[(2S)-3-[2-[(E)-[(2E,4E,6E,8E)-3,7-dimethyl-9-(2,6,6-trimethylcyclohexen-1-yl)nona-2,4,6,8-tetraenylidene]amino]ethoxy-oxidanyl-phosphoryl]oxy-2-[(Z)-octadec-9-enoyl]oxy-propyl] (Z)-octadec-9-enoate | C61 H104 N O8 P | 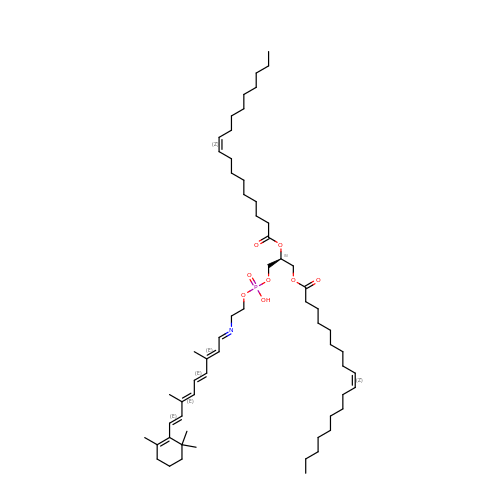DCJYQTYECYRVQM-JOQDOZEYSA-N>[4x]TKPFTLPILTISELTNSRFPIPIEQLYTAPNENNVVQCQNGRCTLDGELQGTTQLLSSAVCSYRGRTVANSGDNWDQNLLQLTYPSGASYDPTDEVPAPLGTQDFSGILYGVLTQDNVSEGTGEAKNAKGVYISTTSGKFTPKIGSIGLHSITENVHPNQQSRFTPVGVAQNENTPFQQWVLPHYAGALALNTNLAPAVAPTFPGEELLFFRSRVPCVQGLRGQDAFIDCLLPQEWVNHFYQEAAPSQADVALIRYVNPDTGRTLFEAKLHRSGFITVSHTGAYPLVVPPNGHFRFDSWVNQFYSLAPM

Human noroviruses (huNoVs), members of the Norovirus genus of the Caliciviridae family, are the leading cause of acute gastroenteritis (AGE) and are associated with almost 20% of all AGE cases worldwide. The major capsid protein (VP1) is composed of a shell (S) domain and a protruding (P) domain, and the P domain is further divided into the P1 and P2 subdomains. The P2 subdomain is the main determinant of NoV diversity, antigenicity, and glycan binding patterns. In conclusion, GII.13/21 huNoVs have developed a novel GBS that interacts with glycans via the common β-Gal through a unique glycan binding mode.

To further explore the structural basis of the observed GII.13 huNoV-glycan interaction, we solved the crystal structure of the GII. SC1065/2016 P domain in complex with Lec disaccharide to a 1.6-Å resolution in the P1211 space group. Lec disaccharide was visible in the (2mFo-DFc) omit difference electron density map, and two sugar rings fitted into the map. The Lec-binding sites are located on the top of each P domain. Eight residues from the P2 domain were involved in binding to the β-Gal of Lec via hydrogen bonding and hydrophobic interactions. Specifically, W298 from the B loop, S357 from the N loop, and N395 and T398 from the T loop formed the bottom region of the binding pocket, and N297 from the B loop, T359 and S360 from the N loop, and N397 from the T loop constituted the edge region of the binding pocket. The β-Gal interacts with the side chains of N297, S357, T359, N395, and N397 through hydrogen bonds, while T398, S360, and W298 form hydrophobic interactions with β-Gal to support the binding outcomes. In contrast, the other saccharide of the Lec disaccharide, N-acetyl-β-glucosamine (β-GlcNAc), points away from the surface of the P dimer and as a result, only a hydrophobic interaction was formed with E396. In addition, the GalNAc formed a hydrogen bond with N396, while the GlcNAc of the mucin core 2 trisaccharide pointed away from the surface of the P dimer without directly participating in the interactions. These structural data show that the GII. P dimer interacts with Lec/core 2 glycans mainly by the common terminal β-Gal.> SSPPVVDTVHGKVLGKFVSLEGFAQPVAIFLGIPFAKPPLGPLRFTPPQPAEPWSFVKNATSYPPMCTQDPKAGQLLSELFTNRKENIPLKLSEDCLYLNIYTPADLTKKNRLPVMVWIHGGGLMVGAASTYDGLALAAHENVVVVTIQYRLGIWGFFSTGDEHSRGNWGHLDQVAALRWVQDNIASFGGNPGSVTIFGESAGGESVSVLVLSPLAKNLFHRAISESGVALTSVLVKKGDVKPLAEQIAITAGCKTTTSAVMVHCLRQKTEEELLETTLKMKFLSLDLQGDPRESQPLLGTVIDGMLLLKTPEELQAERNFHTVPYMVGINKQEFGWLIPQMLMSYPLSEGQLDQKTAMSLLWKSYPLVCIAKELIPEATEKYLGGTDDTVKKKDLFLDLIADVMFGVPSVIVARNHRDAGAPTYMYEFQYRPSFSSDMKPKTVIGDHGDELFSVFGAPFLKEGASEEEIRLSKMVMKFWANFARNGNPNGEGLPHWPEYNQKEGYLQIGANTQAAQKLKDKEVAFWTNLFAK

Human carboxylesterase 1A (hCES1A) was employed as a target enzyme for inhibitory activity (IC50) screening due to its conservative catalytic serine residue. By the analysis of X-ray crystal structure, human CES1A has a serine esterase catalytic triad (Ser-221, His-468, and Glu-354), such catalytic triad is conserved in all mammalian species.. Herein, the halogen effects on the reactivity of the halogenated 2,2,2-trifluoroacetophenones as serine-targeting covalent warheads were investigated. Our results showed that introducing halogen atoms, especially Cl or Br, into the phenyl scaffold would influence the electron density around the ring, which led to different time-dependent inhibition response to the target serine hydrolase (hCES1A).

The covalent interactions were evaluated by nano LC-MS/MS, which offered powerful evidence to support the formation of the covalent adducts and well-explained the time-dependent inhibition of these covalent fragments. Chloro-species compounds F-3 and F-4 were chosen to detect their covalent binding sites on hCES1A. Since the activity of electrophilic warheads and the formation of covalent adducts are related to temperature, we set the incubation conditions at two different temperature points (4 °C and 25°C, respectively). This analysis certainly found several allosteric binding sites, although no expected result of any compound covalently binding to Ser221 at the catalytic cavity of hCES1A. Successfully, the co-crystallography of hCES1A with F-3 and F-4 provided promising covalent binding modes at the catalytic triad. Notably, the co-crystallisation of the parent compound F and hCES1A failed to result in similar covalent interactions. This further proves that the halogen effect may promote the formation of covalent adducts by changing the sensitivity of the electrophilic warhead. The introduction of halogen atoms, particularly chlorine, into the phenyl scaffold enhances the benzocarbonyl reactivity in forming hemiacetal adducts with serine. Co-crystallography analysis not only verified that halogenated molecules preferred to form covalent adducts, but also provided the conformational information for the design of covalent inhibitors targeting to hCES1A protein for the treatment of drug-induced acute enteritis.>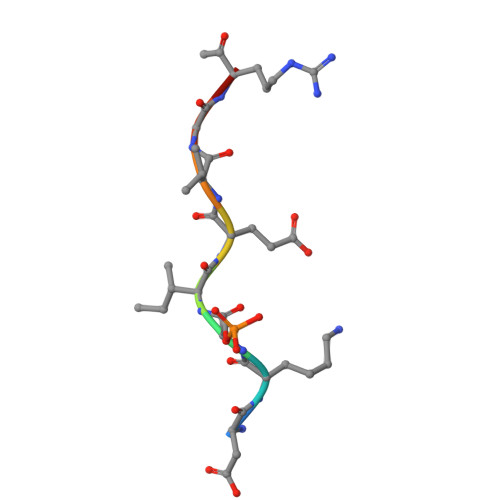 DKSIEVGRX> DEREFDYFILALQWAGTSCRSGGACCPYNGCCKADSPTQFTIHGLRPEYSGGERPSCCTGGSFDPDEIMPFFGKLVEYWPTYRCALEQSCNNRKEILWGQQYEKHGTCASPVIKGEWNYFKKTLKLFMKYNVDKALEDAGIVASNSKMYDLKDIVVAVESAVGARPKLRCDE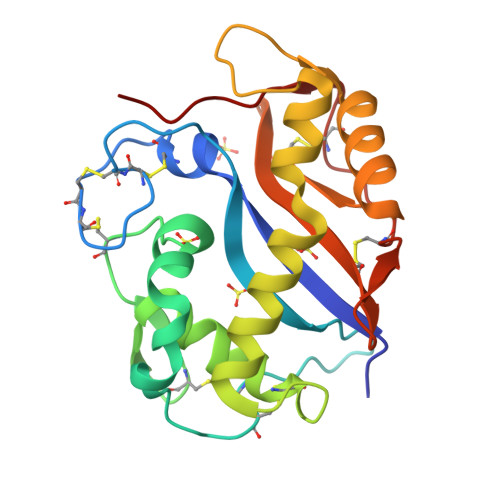EGLVQKLSLCFDKDFKPRDCVQVGSCPRYVSLPEIPD>QNLPQRYIELVVVADHRVFMKYNSDLNTIRTRVHEIVNFINGFYRSLNIHVSLTDLEIWSNEDQINIQSASSDTLNAFAEWRETDLLNRKSHDNAQLLTAIELDEETLGLAPLGTMCDPKLSIGIVQDHSPINLLMGVTMAHELGHNLGMEHDGKDCLRGASLCIMRP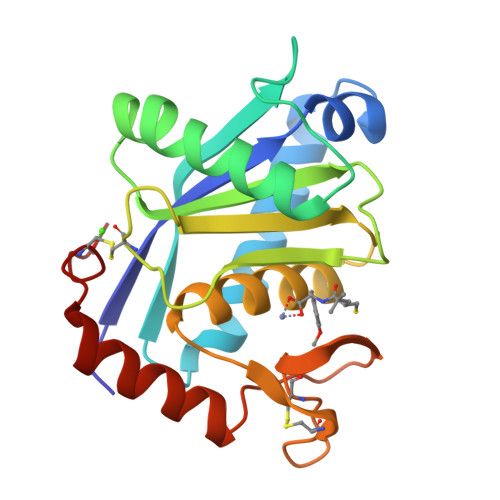GLTKGRSYEFSDDSMHYYERFLKQYKPQCILNKP[2x]5-phenyl-uridine-5'-alpha-d-galactosyl-diphosphate | C21 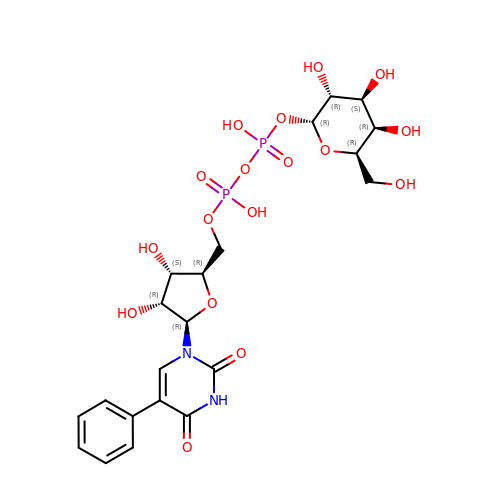H28 N2 O17 P2 | MBQWFWCBPKCMTC-ATMROTIPSA-N>[2x]MSLGATNRLACYSDPADHYSHRVRLVLAEKGVSVQLIDVDPAHLPRKLAEVNPYGSVPTLVDRDLALYESTVVMEYLEERYPHPPLMPVYPVARGNSRLLMHRIQRDWCALADTVLDPRSSE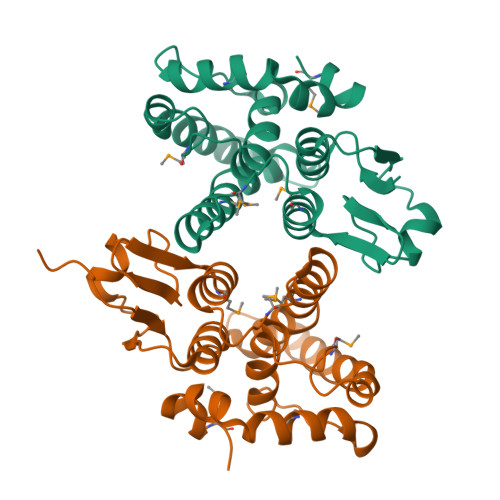AARTEARKALRESLTGVSPLFSEFACFMSDEQSLVDCCLLPILWRLPVLGIELPRQAKPLLDYMERQFAREPFQASLSSVEREMRKLEGHHHHHH>[4x]STPSIVIASAARTAVGSFNGAFANTPAH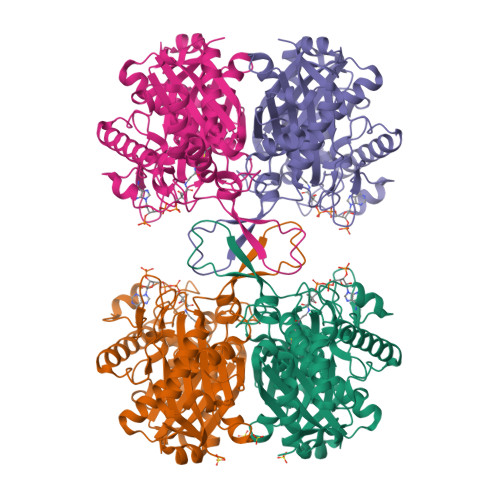ELGATVISAVLERAGVAAGEVNEVILGQVLPAGEGQNPARQAAMKAGVPQEATAWGMNQLAGSGLRAVALGMQQIATGDASIIVAGGMESMSMAPHCAHLRGGVKMGDFKMIDTMIKDGLTDAFYGYHMGTTAENVAKQWQLSRDEQDAFAVASQNKAEAAQKDGRFKDEIVPFIVKGRKGDITVDADEYIRHGATLDSMAKLRPAFDKEGTVTAGNASGLNDGAAAALLMSEAEASRRGIQPLGRIVSWATVGVDPKVMGTGPIPASRKALERAGWKIGDLDLVEANEAFAAQACAVNKDLGWDPSIVNVNGGAIAIGHPIGASGARILNTLLFEMKRRGARKGLATLCIGGGMGVAMCIESL> MEVTVPDALKDRIALKKTARQLNIVYFLGSDTEPVPDYERRLSELLLYLQQFYGKEMQRHGYGARSFGLDIKSPGRVNIIEYKAKNPAAHYPYENGGGWKAAQELDEFFKAHPDRKKSQHTLIIMPTWNDEKNGPDNPGGVPFYGMGRNCFALDYPAFDIKHLGQKTREGRLLTKWYGGMAAALGHGLNLPHNHQTASDGKKYGTALMGSGNYTFGTSPTFLTPASCALLDACEVFSVTPSQQFYEGKPEVEVGDVAISFKGDQILVSGNYKSPQTVKALNVYIQDPPYAVNQDYDAVSFSRRLGKKSGKFSMKIDKKELEGLNNNEFRISLMFILANGLHMQKHFTFHWDALQDYRDGSKSGSGHHHHHH;> GKPRPYSPRPTSHPRPIRV

Here we focus on OgpA from A. muciniphila, a recently discovered O-glycopeptidase that exclusively hydrolyzes the peptide bond N-terminal to serine or threonine residues substituted with an O-glycan. OgpAWT comprises two domains from the N- to the C-terminus: (i) a catalytic domain (residues 25–262) followed by (ii) a β-sandwich domain (residues 263-385). Interestingly, a Zn2+ atom coordinates with the side chains of three histidine residues, H205, H209, and H215, a highly conserved triad among metalloproteases. A glutamate residue, E206, is well-positioned to act as a general base/acid during catalysis.

To obtain the crystal structure of the enzyme-substrate complex, we used a catalytically inactive version of OgpA, in which the residues H205, that coordinates the Zn2+ atom, and E206, the base/acid residue of the reaction, are mutated to alanine (OgpAH205A/E206A). OgpAH205A/E206A-GD-SUB crystallized in the tetragonalI4 space group and diffracted to a maximum resolution of 2.16 Å. The O-glycopeptide 4RPYSPRPT(Gal-GalNAc)SH13 substrate was unambiguously identified in the electron density map. We assume that the full length GD is in the crystal, but no density was observed for the residues 1–3 and 14–19, probably due to conformational flexibility. Strikingly, the GD substrate is inserted as an extra parallel β-strand, relative to the other four strands of the β-sheet comprised in the catalytic domain, in a binding pocket located in the cleft between the N- and C-terminal domains of OgpA. Interestingly, we observe an extensive network of interactions, primarily mediated by hydrogen bonds, between GD’s 8PRPTS12 main chain residues and OgpA’s N315, H215, Y318, and Y236 side chain residues. OgpA mainly interacts with neighboring residues of the glycosylated threonine, suggesting that the enzyme shows a broad range specificity for the peptide backbone. In contrast, the disaccharide Gal-GalNAc is placed in a pocket decorated by four aromatic residues, Y116, F166, W199, and Y236. Finally, in the OgpAH205A/E206A-GD-SUB, Thr-S1’ subsite is wide and Thr-P1’barely interacts with OgpA. However, the Gal and GalNAc moieties of the O-glycan attached to this residue closely interacts with the enzyme’s subsites G1’ and G2’ via hydrogen bonding, hydrophobic and CH–π interactions, respectively.>LVYSEAGPVALWLARVRWLVILILTGMVTSSILQGFESVLEAVTALAFYVPVLLGTGGNTGNQSATLIIRALATRDLDLRDWRRVFLKEMGVGLL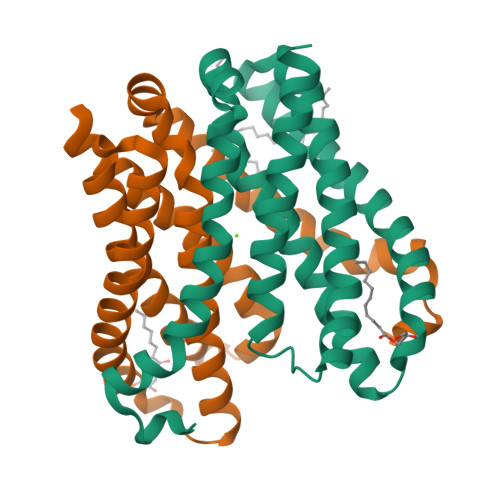LGLTLSFLLVGKVYWDGHPLLLPVVGVSLVLIVFFANLVGAMLPFLLRRLGVDPALVSNPLVATLSDVTGLLIYLSVARLLLEA[2x]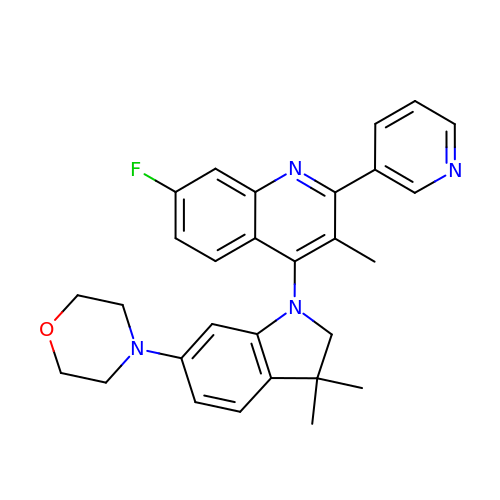4-[3,3-dimethyl-6-(morpholin-4-yl)-2,3-dihydro-1H-indol-1-yl]-7-fluoro-3-methyl-2-(pyridin-3-yl)quinoline | C29 H29 F N4 O | IGGNGGDYLDZKTR-UHFFFAOYSA-N>[2x]SNVRATYTVIFKNASGLPNGYDNWGWGCTLSYYGGAMIINPQEGKYGAVSLKRNSGSFRGGSLRFDMKNEGKVKILVENSEADEAFEVETISPSDEYVTYILDVDFDLPF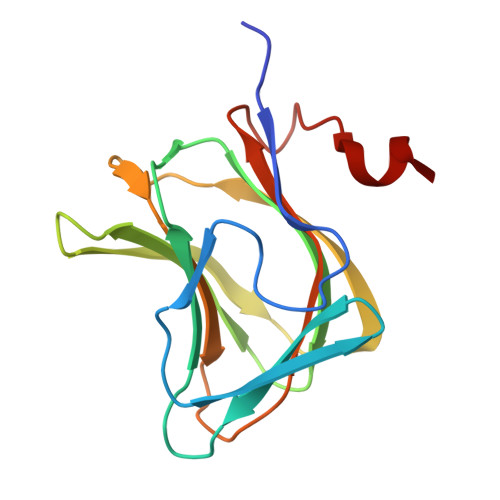DRIDFQDAPGNGDRIWIKNLVHSTGSADDFVDPINLHHH> AMKDHKFWRTQPVKDFDEKVVEEGPIDKPKTPEDISDKPLPLLSSFEWCSIDVDNKKQLEDVFVLLNENYVEDRDAGFRFNYTKEFFNWALKSPGWKKDWHIGVRVKETQKLVA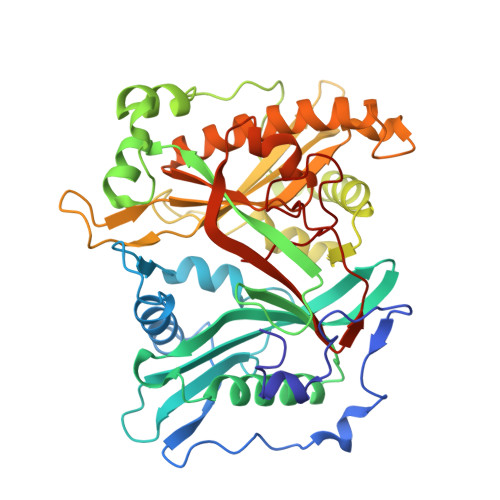FISAIPVTLGVRGKQVPSVEINFLCVHKQLRSKRLTPVLIKEITRRVNKCDIWHALYTAGIVLPAPVSTCRYTHRPLNWKKLYEVDFTGLPDGHTEEDMIAENALPAKTKTAGLRKLKKEDIDQVFELFKRYQSRFELIQIFTKEEFEHNFIGEESLPLDKQVIFSYVVEQPDGKITDFFSFYSLPFTILNNTKYKDLGIGYLYYYATDADFQFKDRFDPKATKALKTRLCELIYDACILAKNANMDVFNALTSQDNTLFLDDLKFGPGDGFLNFYLFNYRAKPITGGLNPDNSNDIKRRSNVGVVML> MSLNYEESNLIVFGVGFDGTTSNRPGARFASSSMRKEFYGLETYSPFLDLDLEDYNICDYGDLEISV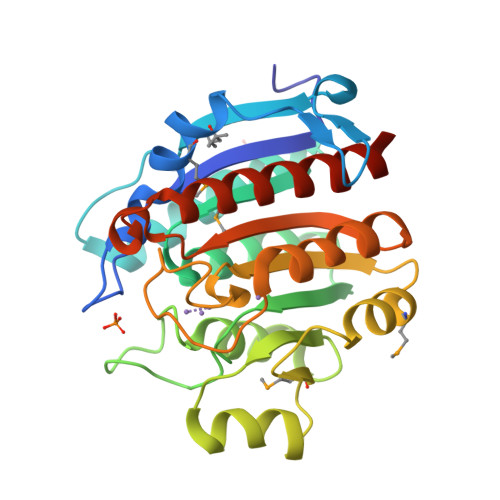GSTEQVLKEIYQETYKIVRDSKVPFMIGGEHLVTLPAFKAVHEKYNDIYVIHFDAHTDLREEYNNSKNSHATVIKRIWDIVGDNKIFQFGIRSGTKEEFKFATEEKHTYMEIGGIDTFENIVNMLNGKNIYLTIDLDVLDASVFPGTGTPEPGGVNYREFQEIFKIIKNSNINIVGCDIVELSPDYDTTGVSTVIACKILRELCLIISDKIKEGHHHHHH> MSLAKVWTYASWIPRGIPKAMANELSSAAAALAHPEAIARVAQLESQGKNPYRVARAEFWQMYLACWPYRFRNTVVEWETCKAKVLKGSVDLQDIVDLLYLLAWAYLFWILGEIYGRGSLYGYRFDGEIHRQEAQNVILYKEKEAQEMAVVMEKLEKEIQEWLKTMEQE;> MPGGGTIRFWREKLEGYKKYHQIVKTIKMVTLAKYRQTVVRTRVRDQTLRYTRKALDAKTQDDQEVIEKSECLLYVPITTNRGSCGALNTNMVRYLQEVENPKMTIISVGKKALDAMTKVFQDTYRRTILNDMKQAMSFQFAAYVLEHMNTVPWDRAQIVYNRYHGAASQKLAIFNLPKFEDWKQKLEEDSAGDGKIEEDGLLQSLPMKTALGELEETAVEDFYNFHSCLAVLNAVSENELSEYAARIVAVENQLGNITGLMQLADYTYNKTRKELITAELLEIIGTMTAMHAGKKVGLKKTEFWK;> MRASRTLLLSVSRFMRQDPRKFFPDNGFRFFDGPEDSFGDGNIPAQIILTLTRQDEFILKQEPVAAITIRTNEGEMGVLAGHEYTVQQLAPGILEVEYEGGKKDQYVISGGFAHVNDTGVVDINTVEAVPLEEIDHEKLAKALEEARAKSQSPDEAVRIQGEIALEIFEPLEAALH;> MSWRDAGISYLRYLSIVTRCIHEVQKEGPLLTKNVRFSTIGWKSLYLDHGATKEYTAIPAELEKIPENQVAQQHHA;>MQRGSSITKVVRRAALARSTRNAAIAYEVTVNGANLIGAGMAASGVGVPAIGVAMCFSSYMLAAARQPNMSAKLLPYCILGFALSEALALFTLLIALLELFVFS[10x]

The mitochondrial ATP synthase is a membrane protein complex that generates most of the ATP in eukaryotic cells. The translocation of protons through the membrane-bound Fo part, mediated by subunit a, drives the rotation of a membrane-embedded c-ring and the attached central stalk, which together form the rotor. The torque of the rotor against the stator subunits induces conformational changes in the (αβ)3 headpiece, thereby triggering catalysis. To reveal how the mitochondrial ATP synthase is modulated by lipids and organised into a dimer shaping discoid cristae in Euglenozoan mitochondria, we determined the structure of the ATP synthase dimer from E. gracilis.

Symmetry expansion of the pseudo-C2-symmetric dimer particles was used to classify individual F1/c-ring monomers into rotational states 1, 2 and 3 (named according to bovine nomenclature; Zhou et al., 2015) and resolve structures at 3.0- to 3.9 Å resolution. Using masked refinement, maps of the membrane region, the rotor and the peripheral stalk tip were refined to 2.8 and 3.3 and 3.8 Å resolution, respectively, enabling the construction of atomic models (Figure 1—figure supplements 1–2). The C-terminal helix of euglenozoa-specific ATPEG1 (H5EG1) extends 50 Å from the membrane region into the lumen, where it interacts with the N-terminal extensions of subunit c, which together form a ten-stranded β-barrel protruding ~20 Å into the lumen. The N-terminal residues of subunit c (A24, I25) form a hydrophobic interface with hydrophobic residues (M148, M152, L155, I159, L163) of the amphipathic ATPEG1 helix. The position of the lumenal H5EG1 on the c-ring β-barrel remains largely unchanged in all three rotational states, suggesting a mechanism of transient rotor-stator interaction during c-ring rotation. The extensions of OSCP and subunit γ are conserved in Kinetoplastida, suggesting that the observed interaction is a structural feature of euglenozoan ATP synthases. Together, the matrix-exposed subunit γ/OSCP interactions and lumenal ATPEG1/c-ring contacts pin the F1/c-ring-complex to the stator, likely providing additional stability.> GSHMKNATFYLLDNDTTVDGLSAVEQLVCEIAAERWRSGKRVLIACEDEKQAYRLD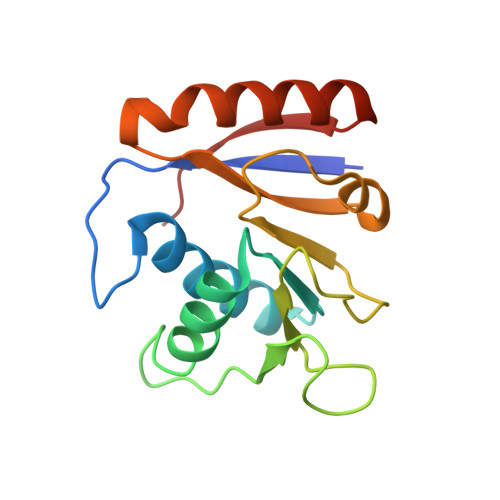EALWARPAESFVPHNLAGEGPRGGAPVEIAWPQKRSSSRRDILISLRTSFADFATAFTEVVDFVPYEDSLKQLARERYKAYRVAGFNLNTATWK> KVEQAVETEPEPELRQQTEWQSGQRWELALGRFWDYLRWVQTLSEQVQEELLSS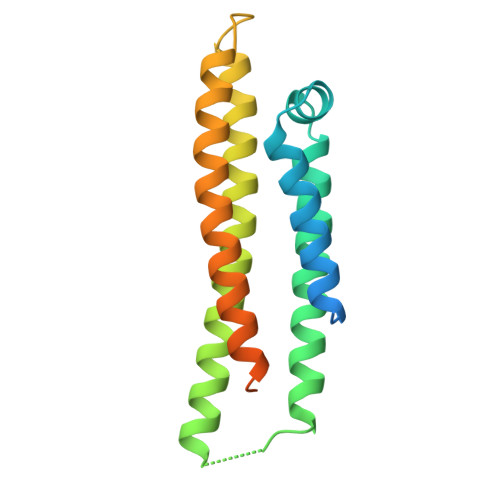QVTQELRALMDETMKELKAYKSELEEQLTPVAEETRARLSKELQAAQARLGADMEDVRGRLVQYRGEVQAMLGQSTEELRVRLASHLRKLRKRLLRDADDLQKRLAVYQAGAREGAERGLSAIRERLGPLVEQGRVR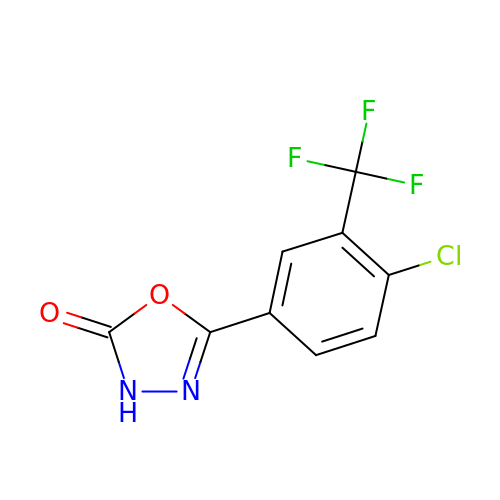5-[4-chloranyl-3-(trifluoromethyl)phenyl]-3~{H}-1,3,4-oxadiazol-2-one | C9 H4 Cl F3 N2 O2 | SBBOPUCCCOEMDA-UHFFFAOYSA-N1-(2,3-dihydro-1-benzofuran-5-yl)methanamine | C9 H11 N O | 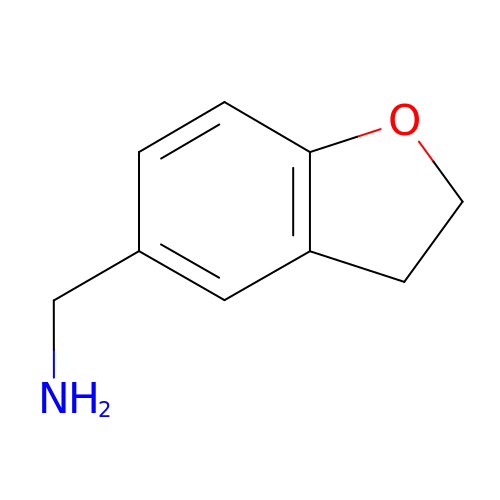WQXWNTPLZFVZNX-UHFFFAOYSA-N>[2x]MLYNMDERFEIKDIVAREVIDSRGNPTVEVEVITKGNGYGSAIVPSGASTGTHEALELRDKEKRFGGKGVLMAVENVNSIIRPEILGYDARMQREIDTIMI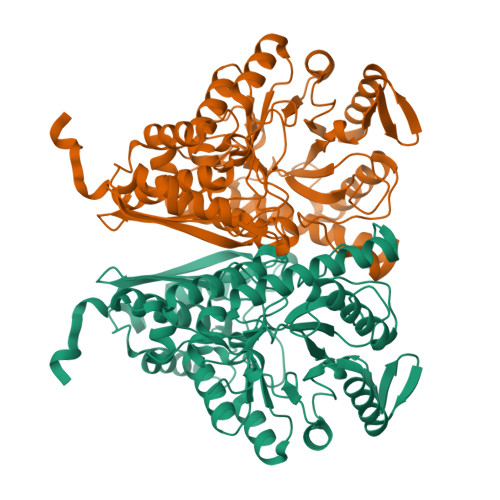ELDGTPNKSRLGANAILAVSLAVAKAAAATAKIPLYKYLGGFNSYVMPVPMMNVINGGKHAGNDLDLQEFMIMPVGATSISEAVRMGSEVYHVLKNVILEKYGKNAVNVGDEGGFAPPLKTSREALDLLTESVKKAGYEDEVVFALDAAASEFYKDGYYYVEGKKLTREELLDYYKALVDEYPIVSIEDPFHEEDFEGFAMITKELDIQIVGDDLFVTNVERLRKGIEMKAANALLLKVNQIGTLSEAVDAAQLAFRNGYGVVVSHRSGETEDTTIADLSVALNSGQIKTGAPARGERTAKYNQLIRIEQELGLSKYAGRNFRCPF> GLPVCGETCVG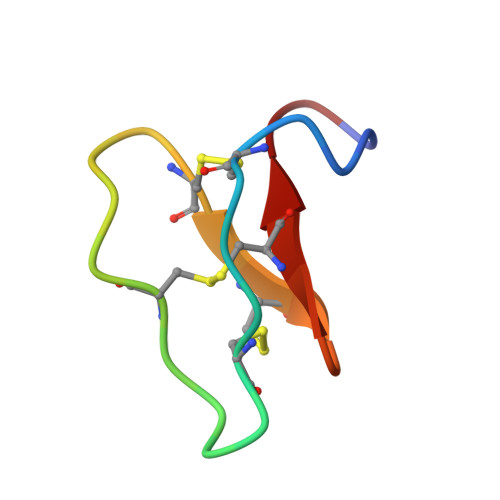GTCNTPGCTCSWPACTRN;> GLPVCGETCVGGTCNTPGCTCSWPVCTRN> AKATTSVNYAANLDKRLPELPEGANRAQILESTWSTEFKVYDSFGEAHELQIDFARVPGEVNAWRATVNVDPT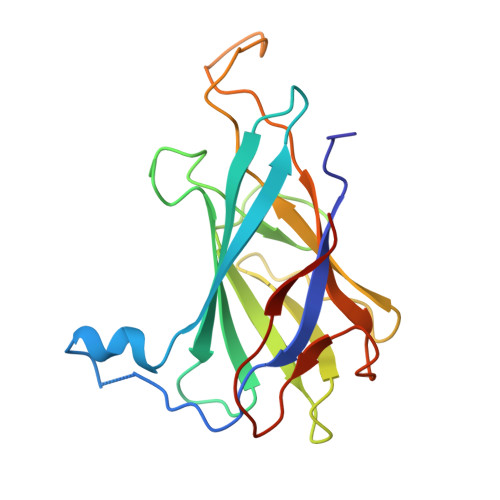NADATATRVGIGTTDGVQNSFIVRFDNNGHLASVTDTAGNVTSPAGQVLVQISYNVVGANPDEAGAPTRHTFDVNLGEIGTSKNTITQFSDKSTTKAYEQDGYT> MDEAVGDLKQALPCVAESPTVHVEVHQRGSSTAKKEDINLSVRKLLNRHNIVFGDYTWTEFDEPFLTRNVQSVSIIDTELKVKDSQPIDLSACTVALHIFQLNEDGPSSENLEEETENIIAANHWVLPAAEFHGLWDSLVYDVEVKSHLLDYVMTTLLFS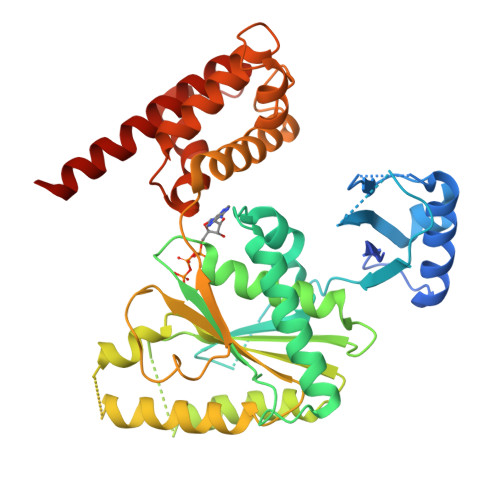DKNVNSNLITWNRVVLLHGPPGTGKTSLCKALAQKLTIRLSSRYRYGQLIEINSHSLFSKWFSESGKLVTKMFQKIQDLIDDKDALVFVLIDQVESLTAARNACRAGTEPSDAIRVVNAVLTQIDQIKRHSNVVILTTSNITEKIDVAFVDRADIKQYIGPPSAAAIFKIYLSCLEELMKCQIIYPRQQLLTLRELEMIGFIENNVSKLSLLLNDISRKSEGLSGRVLRKLPFLAHALYVQAPTVTIEGFLQALSLAVDKQFEERKKLAAYI>[4x]SNAVFGVKEWECEVLSNKNVSTFIKEFVVKLPEGETMNFKSGSYAQIKIPKYNIRYADYDIQDRFRGDWDKMDAWSLTCKNEEETVRAYSMANYPAEGNIITLNVRIATPPFDRAANKWKAGIKPGISSSYIFSLKPGDKVMMSGPYGDFHIQDTDAEMLYIGGGAGMAPLRAQILHLFRTLKTGRKVSYWYGARSKNEIFYEEDFREIEREFPNFKFHIALSDPQPEDNWTGYVGFIHQVIY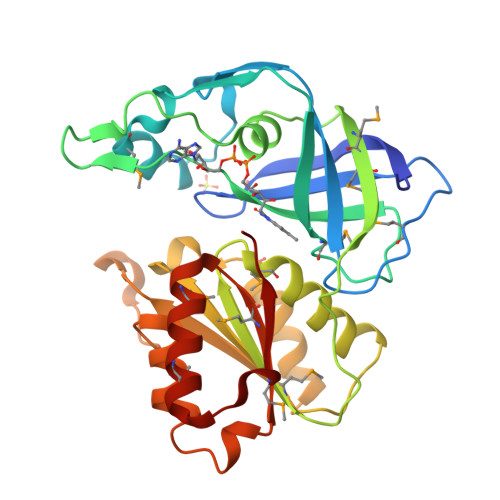DNYLKDHDAPEDIEYYMCGPGPMANAVKGMLENLGVPRNMLFFDDFG> MKILYKKILNLELWHDFYLGQPNTPGSLPNNYDISRTLALVPTQECLRVLANLRWVFRPQLYGASLFANVNAAPSGQFPTIFPIDRVY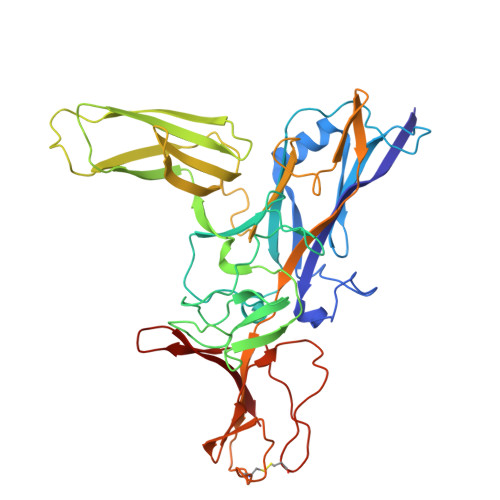RLTFWLVVSDRYFANFTNLSLINSRNQIYYFSNLSGNEGHALFLTQPLSAYTTNNEYQLGQLVTHADKTLESLTYQGNATNIPNPSDWDSLPASQYVSELDHLPRQGTYRTQVITNANPDNTYNFTLVNTNEQESWAIDVIVPDTHKSGEPFSTSLNFVGQTPGHYRLLENDTQVAEFVLVDNSLPEAFALVEVILNPELVPSAFSLLQASAGQTFIQPKTYVIRFKNRATRWRYRYEQPHGCSAANLPSYFNLIDTHTYATARPIGLRQRPDSLLNDCQDRPLPAPSITLIQPETDGSQRIARIFSDIYL2-[(1-methoxy-7-naphthalen-2-yloxy-4-oxidanyl-isoquinolin-3-yl)carbonylamino]ethanoic acid | C23 H18 N2 O6 | 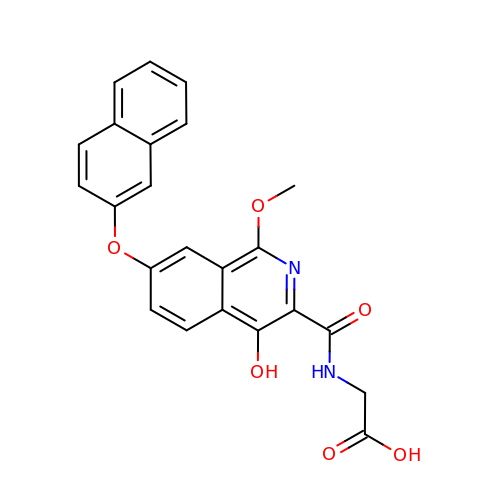OJFUTFNCRATZLZ-UHFFFAOYSA-N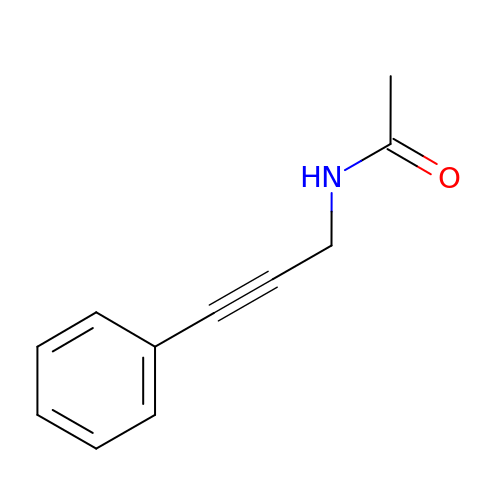N-(3-phenylprop-2-yn-1-yl)acetamide | C11 H11 N O | MEDMJWLHQZDCBX-UHFFFAOYSA-N>AKYYNEPCHTFNEYLLIPGLSTVDCIPSNVNLSTPLVKFQKGQQSEINLKIPLVSAIMQSVSGEKMAIALAREGGISFIFGSQSIESQAAMVHAVKNFKDSQKRYLVGAGINTRDFRERVPALVEAGADVLCIDSSDGFSEWQKITIGWIREKYGDKVKVGAGNIVDGEGFRYLADAGADFIKIGIGGGSICITREQKGIGRGQATAVIDVVAERNKYFEETGIYIPVCSDGGIVYDYHMTLALAMGADFIMLGRY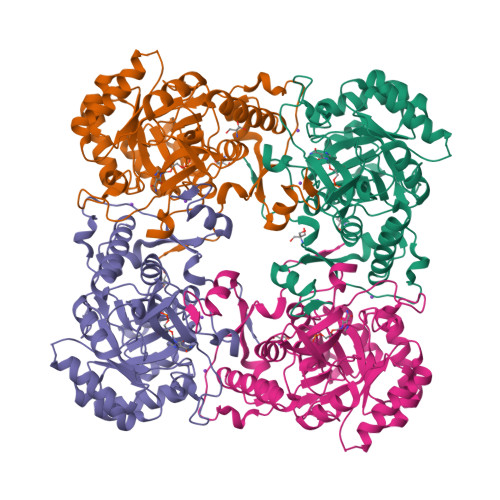FARFEESPTRKVTINGSVMKEYWGEGSSRARNWQRYDLGGKQKLSFEEGVDSYVPYAGKLKDNVEASLNKVKSTMCNCGALTIPQLQSKAKITLVSSVSIVEGGAHDVIVKDRINDYHPK[4x]> GRPFVEMYSEIPEIIHMTEGRELVIPCRVTSPNITVTLKKFPLDTLIPDGKRIIWDSRKGFIISNATYKEIGLLT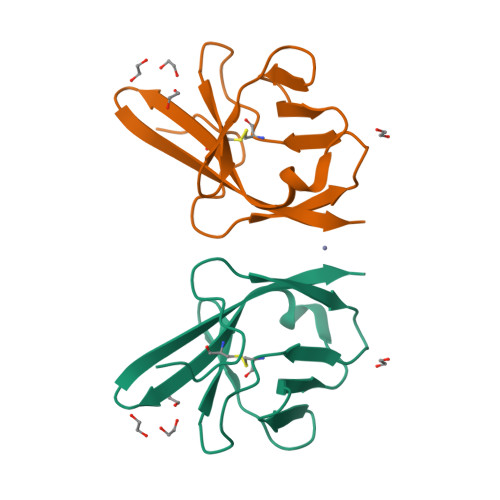CEATVNGHLYKTNYLTHRQ Functional ParMRC plasmid segregation systems comprise an actin-like polymerizing motor (ParM), a centromere-like specific DNA sequence (parC), and an adaptor protein (ParR), which attaches a plasmid, via the parC, to each end of the growing ParM filament or filament bundle. Thus, the force generated from ParM polymerization is harnessed for plasmid segregation. Here we investigated the ParMRC cassette from pCBH, a 257 kb plasmid that carries the botulinum neurotoxin type B. This ParMRC cassette is also found on other C. botulinum plasmids, such as pCLK (267 kb) and pRSJ2_3 (245 kb), which encode neurotoxin types A and F, respectively. Despite the similarities to actin, pCBH ParM is a genuine ParM, since it has a closed β-barrel, a feature that is missing from actin and MreB structures.

Due to this complexity, the helical parameters were determined by cryoelectron tomography (axial rise 5.2 nm, twist −50.1°). These parameters refined to a distance 5.03 nm and twist −50.4° with the cryoEM data. Helical averaging of the cryoEM density, from each cross-section of the filament, based on these parameters led to a 4.7 Å map for the entire filament. The pCBH ParM filament has a diameter of 26 nm and of consists of 15 loosely associated, left-handed helical, single strands arranged in three layers in cross-section. At the center there is a single straight helical strand. This is surrounded by an intermediate layer of six interacting twisted helical strands that have the opposite polarity (antiparallel) to the central strand. The outer layer comprises eight non-interacting helical strands, which have a different twist and polarity (antiparallel) to the intermediate layer strands but have the same polarity (parallel) as the central strand. The 15 strands are in register in each cross-section despite having different radii and path lengths. The major type of inter-strand interaction occurs between complimentary basic and acidic patches on the protomers. Prominent in the acidic patch are two acidic loops (A1 loop and A2 loop), which adopt different positions across the basic surfaces of neighboring protomers in a lateral cross-section, allowing for multiple types of inter-strand contacts.

>MNKYTIAIDLGYGQIKGINQDNKRVIFPSIISSGKDRSLDTFFNSIDNIVDNIHVKILDEYFNEKEYFVGELAKRQPSNSSFINRDNKINSEENKVLLATALGLLIPNDLPNDTKIHIVTGLPLEHFIKQKQALNDMLKDFEHTIKFVDHNFSRNIKFEESNITLFPQGAGAIFSKINNDISSLLIKETFIGLIDVGFKTTDIVVFRINKDKEPVFEQEMSATLDGLGMINIYNTMDKAFTDNSRDGSKLNTEQLMLLCEEGKIFFKGDYIDLKKDLIKARKTLSTNIINKADGLWGSRKNSFNSIMIAGGGGKVLYNHLKLIEPNMCQLIDNPEFANAIGYLEFGKQF[30x]> MGKTNDWLDFDQLAEEKVRDALKPPSMYKVILVNDDYTPMEFVIDVLQKFFSYDV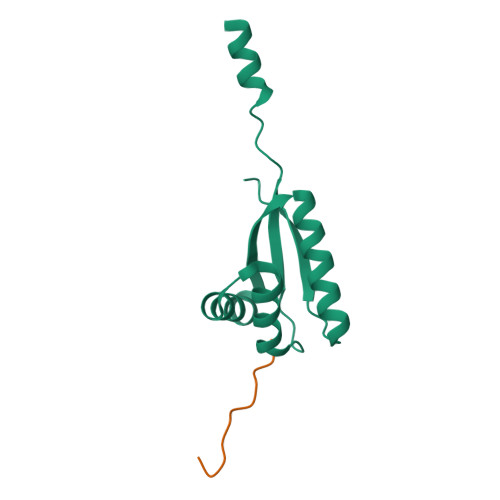ERATQLMLAVHYQGKAICGVFTAEVAETKVAMVNKYARENEHPLLCTLEKAGA;> LVKSKATNLLY> DYKDDDDAMGRSHTITMTTTSVSSWPYSSHRMRFITNHSDQPPQNFSATPNVTTCPMDEKLLSTVLTTSYSVIFIVGLVGNIIALYVFLGIHRKRNSIQIYLLNVAIADLLLIFCLPFRIMYHINQNKWTLGVILCKVVGTLFYMNMYISIILLGFISLDRYIKINRSIQQRKAITTKQSIYVCCIVWMLALGGFLTMIILTLKKGGHNSTMCFHYRDKHNAKGEAIFNFILVVMFWLIFLLIILSYIKIGKNLLRISKRRSKFPNSGKYATTARNSFIVLIIFTICFVPYHAFRFIYISSQLNVSSCYWKEIVHKTNEIMLVLSSFNSCLDPVMYFLMSSNIRK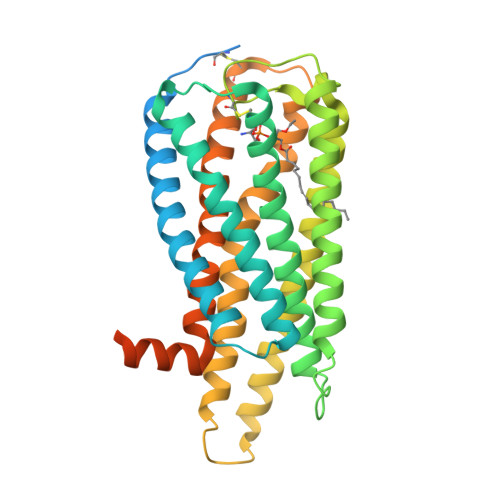IMCQLLFRRFQGEPSRSESTSEFKPGYSLHDTSVAVKIQSSSKSTENLYFQ> PISPIETVPVKLKPGMDGPKVKQWPLTEEKIKALVEICTEMEKEGKISKIGPENPYNTPVFAIKKKDSTKWRKLVDFRELNKRTQDFWEVQLGIPHPAGLKKKKSVTVLDVGDAYFSVPLDEDFRKYTAFTIPSINNETPGIRYQYNVLPQGWKGSPAIFQSSMTKILEPFKKQNPDIVIYQYMDDLYVGSDLEIGQHR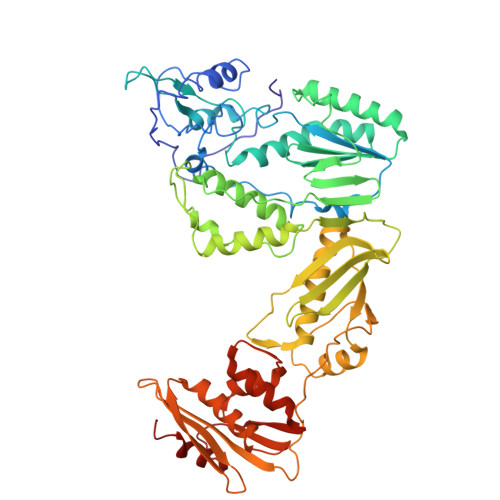TKIEELRQHLLRWGLTTPDKKHQKEPPFLWMGYELHPDKWTVQPIVLPEKDSWTVNDIQKLVGKLNWASQIYPGIKVRQLCKLLRGTKALTEVIPLTEEAELELAENREILKEPVHGVYYDPSKDLIAEIQKQGQGQWTYQIYQEPFKNLKTGKYARMRGAHTNDVKQLTEAVQKITTESIVIWGKTPKFKLPIQKETWETWWTEYWQATWIPEWEFVNTPPLVKLWYQLEKEPIVGAETFYVDGAANRETKLGKAGYVTNKGRQKVVPLTNTTNQKTQLQAIYLALQDSGLEVNIVTDSQYALGIIQAQPDKSESELVNQIIEQLIKKEKVYLAWVPAHKGIGGNEQVDKLVSAGIRKIL> TPYDPLTLWTTPDPPPNCSLIQELDAKLTLCLTKNGSIVNGIVSLVGVKGNLLNIQSTTTTVGVHLVFDEQGRLI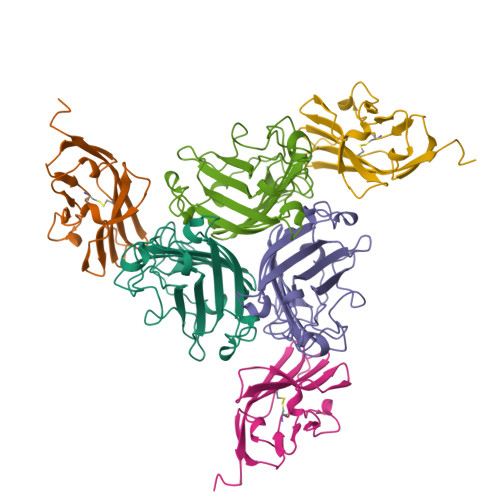TSTPTALVPQASWGYRQGQSVSTNTVTNGLGFMPNVSAYPRPNASEAKSQMVSLTYLQGDTSKPITMKVAFNGITSLNGYSLTFMWSGLSNYINQPFSTPSCSFSYITQE;> GITTPEEMIEKAKGETAYLPCKFTLSPEDQGPLDIEWLISPADNQKVDQVIILYSGDKIYDDYYPDLKGRVHFTSNDLKSGDASINVTNLQLSDIGTYQCKVKKAPGVANKKIHLVVLVKPSGA> APKVVKFSYMWTINNFSFCREEMGEVIKSSTFSSGANDK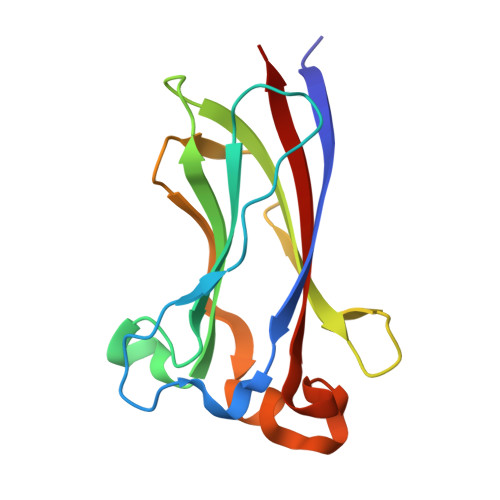LKWCLRVNPKGLDEESKDYLSLYLLLVSCPKSEVRAKFKFSILNAKGEETKAMESQRAYRFVQGKDWGFKKFIRRDFLLDEANGLLPDDKLTLFCEVSVVQD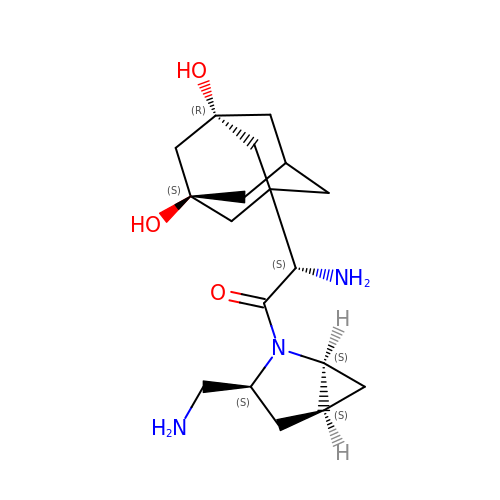(2S)-2-amino-1-[(1S,3S,5S)-3-(aminomethyl)-2-azabicyclo[3.1.0]hexan-2-yl]-2-[(1r,3R,5S,7S)-3,5-dihydroxytricyclo[3.3.1.1~3,7~]decan-1-yl]ethan-1-one | C18 H29 N3 O3 | NFCLGRKAEZJOPE-KAARGAEXSA-N>GPHMSELREDIQTKGKEVENFEKNL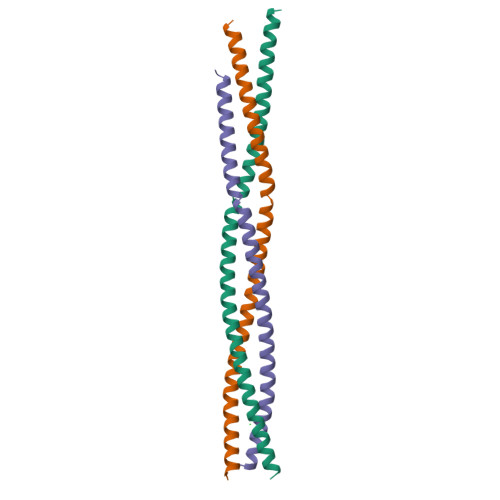EECITRITNTEKCLKELMELKTKARELREECRSLRSRCDQLEERVSAAEDEINEIKREGKFREKRIKRNEQSLQEIWDY[6x]> GSNFCDSKCKLRCSKAGLADRCLKFCGICCEECKCVPSGTYGNKHECPC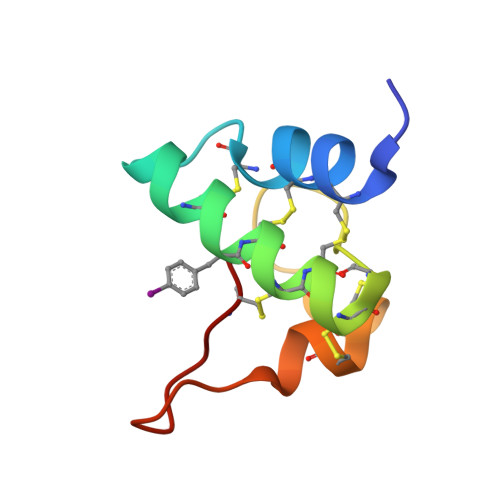YRDKKNSKGKSKCP One such nuclease, NucA (Gbs0661) from S. agalactiae (henceforth referred to as GBS_NucA), has been shown to degrade NETs and to improve infection persistence in the host. GBS_NucA is thought to be a sequence-nonspecific DNA/RNA nuclease with endonucleolytic and exonucleolytic activity. Although this family of nucleases share a common ββα metal-finger catalytic core and reaction mechanism, their global structures, localization and regulatory mechanisms can vary widely. As a starting point for such development, we have determined high-resolution X-ray crystal structures of GBS_NucA with and without bound magnesium ion and compared them with those of other ββα metal-finger nucleases.

GBS_NucA was also crystallized in space group P63 in the presence of a divalent Mg2+ ion and a putative substrate DNA, although there was no visible electron density for the DNA. Asn179 is the only residue to directly interact with the metal. An intricate network of putative hydrogen-bonding interactions links the metal in the active center through Asn179 to the distally located Gln180 and His142, using Asp145 as the intermediary. The most significant difference is observed in the ordering of the coil between β-strands 4 and 5 of molecules A and B in the P63 crystal form. This is the first reported structure of a Streptococcus sp. nuclease in which this loop is ordered. Residues Arg116–Asp118 along this loop form a short α-helix (henceforth referred to as α-helix S), although there are no such indications of helical propensity in Arg116–Asp118 in the P1 crystal form. Given that this coil is entirely disordered in the P1 crystal form and is incomplete in molecules C and D of the P63 crystal form, we hypothesize that it is highly mobile in the absence of a DNA substrate. Since residues along this loop in EndA (Arg127/Lys128) have been shown to strongly influence DNA binding and these residues appear to be conserved in GBS_NucA (Arg116/Arg117), this region might also act as a substrate-binding loop in this enzyme. Since Asn179 is the only protein side chain directly chelating the hydrated divalent Mg2+ ion in the active site, these results provide confirmation that the plasmid conversion and SRED assays are performing as expected.

>[4x]GSAAASSVDTSQEFQNNLKNAIGNLPFQYVNGIYELNNNQTNLNADVNVKAYVQNTIDNQQRPSTANAMLDRTIRQYQNRRDTTLPDANWKPLGWHQVATNDHYGHAVDKGALIAYALAGNFKGWDASVSNPQNVVTQTAHSNQSNQKINRGQNYYESLVRKAVDQNKRVRYRVTPLYRNDTDLVPFAMHLEAKSQDGTLEFNVAIPNTQASYTMDYATGEITLN~{N}-(5-ethyl-6-oxidanylidene-benzo[b][1,4]benzothiazepin-2-yl)-2-(4-fluorophenyl)ethanamide | 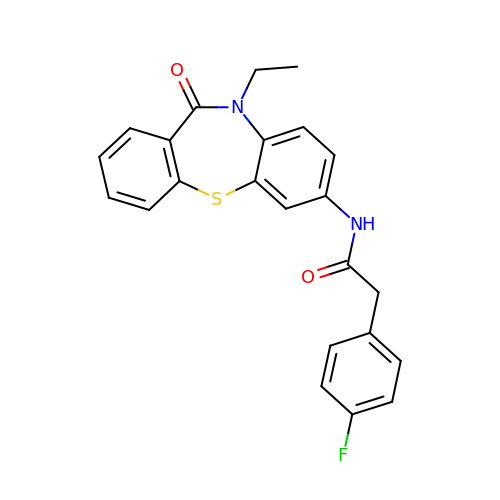C23 H19 F N2 O2 S | HMFFZASNCXIJTL-UHFFFAOYSA-N>RPNHTIYINNLNEKIKKDELKKSLHAIFSRFGQILDILVSRSLKMRGQAFVIFKEVSSATNALRSMQGFPFYDKPMRIQYAKTDSDI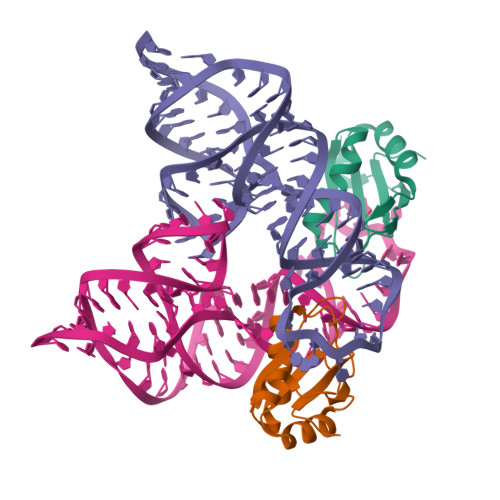IAKM[2x]> MAQDWQLSELLENLHADVQHKLTTVRKSFKHSVVKGDGAENVWVDLFNQYLPERYRASRAFVVDSENQFSEQIDVVIYDRQYSPFIFHYAEQLIIPAESVYAVFEVKQTLNKQHIDAARKKVA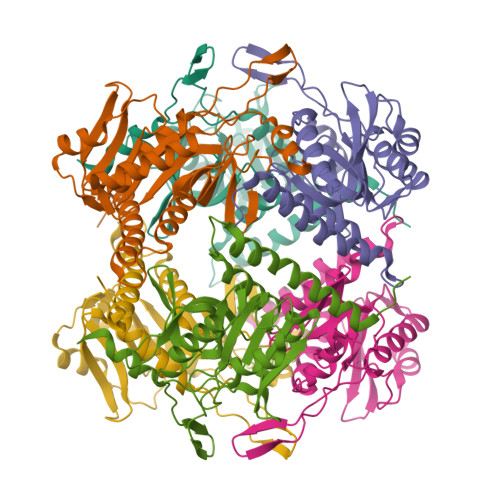SVRALHRTSLPIPHAGGVHSPRELIGIIGGLLTLENELKIPDTLMGHLDHDKADKGMLNIGCAADDCFFYYDNDHQRMQVMQHKKATTAFLFELLSQLQKCGTVPMIDIHAYGKWLTPRISE> GAMESEQFLTELTRLFQKCRTSGSVYITLKKYDGRTKPIPKKGTVE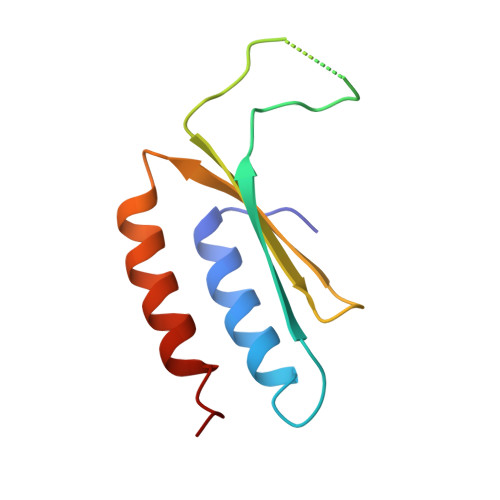GFEPADNKCLLRATDGKKKISTVVSSKEVNKFQMAYSNLLRANMDGLK The cap open reading frame encodes three viral proteins (VP), VP1, VP2, and VP3, that form the capsid shell. The AAV capsid is comprised of a total of 60 VP monomers. All AAV capsids exhibit T = 1 icosahedral symmetry, but only the shared C-terminal VP3 region has been resolved, while the extended N-termini of VP1 and VP2 are intrinsically disordered. Within VP3, the central core motif is an eight-stranded β-barrel (jellyroll motif) formed by two sets of four antiparallel β-sheets (βBIDG and βCHEF), with an additional βA-strand and one α-helix.

For AAVpo.1 and AAVpo.6 capsid structures were generated from 512,823 and 539,729 particles, resulting in final maps with resolutions of 1.79 and 1.77 Å, respectively. The amino acid sequence could be readily built to the density maps, starting from amino acid 198 for AAVpo.1 and 217 for AAVpo.6 which is comparable to all previous AAV capsid structures. The lower residue number for AAVpo.1 is due to large deletions in the VP1/2 common region. Amongst the AAVs compared, AAV5 and AAVpo.1 share the highest percentage of aligned residues (99%) and lowest overall Cα-RMSD value. Both AAVs share very similar loop conformations in VR-I, -VII, the HI-loop, and VR-IX. AAVpo.1 shows a ~2-fold higher transduction efficiency in Lec-2 cells as compared to Pro-5, indicating a preference for terminal galactose. This behavior is surprising, considering the high sequence identity and structural similarity of AAVpo.1 to AAV5. The sialic acid binding site on the AAV5 capsid has been identified previously and the substitutions of methionine (M) 569 to valine (V) and leucine (L) 587 to threonine (T) on the AAV5 capsid resulted in the loss of sialic acid binding ability. These residues are not conserved in the AAVpo.1 capsid explaining its inability to bind sialic acid compared to AAV5. For the AAVpo.1 capsid, this is not surprising as there is little sequence conservation with the AAV9 residues around the 2-fold region. In contrast, AAVpo.1 is not recognized by mAb1-6 and weakly by mAb2-7.

>[60x]MSAGGGSPLGDNNQGADGVGNASGDWHCDSTWMGDRVITKSTRTWVLPSYNNHQYLEIHSGSVDGSNANAYFGYSTPWGYFDFNRFHSHWSPRDWQRLVNNYWGFRPRSLKVKIFNIQVKEVTTQDGTTTIANNLTSTVQVFTDNDYQLPYVIGNGTEGCLPAFPPQVFTLPQYGYATLNRNNTDDPTERSSFFCLEYFPSKMLRTGNNFEFTYSFEEVPFHCSFAPSQNLFKLANPLVDQYLYRFVSTDTSGNLQFQKNLKARYANTYKNWFPGPMCRTQGWYTSAGTYNNKGVANFDTSNKMELEGASYQVNPQPNGMTNTLQDSNKYALENTMIFNAQNAPPGTTSLYQENNLLITSESETQPVNRLAYNTGGQVSNNNQNSNTHPTVGVYNHQEVLPGSVWMDRDVYLQGPIWAKIPETGAHFHPSPAMGGFGLKHPPPMMLIKNTPVPSNVAAFSDVPVKSFITQYSTGQVTVEIEWELKKENSKRWNPEIQYTNNYNNPTFVDFAPDTSGEYRTTRAIGTRYLTRPL> SWQTYVDEHLMCDIEGTGQHLASAAIFGTDGNVWAKSSSFPEFKPDEINAIIKEFSEPGALAPTGLFLAGAKYMVIQGEPGAVIRGKKGAGGICIKKTGQAMVF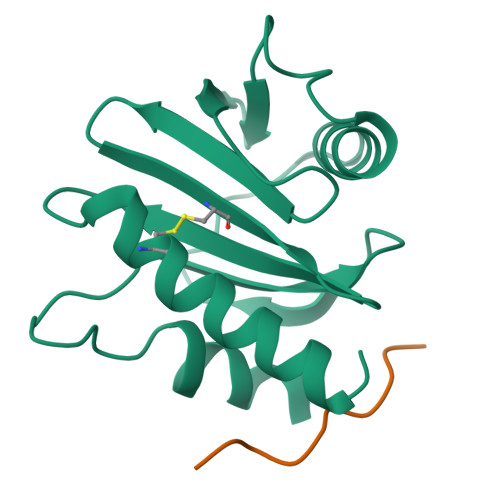GIYEEPVNPGQCNMVVERLGDYLVDQGM;> PPPPPPPPPP The eukaryotic translation initiation factor 4E (eIF4E) protein is a vital component of the cap-dependent mechanism for mRNA translation. It binds the 7-methylguanosine (m7G) cap structure present at the 5′ end of mRNA molecules and recruits it as part of the eIF4F assembly which also includes two other partner proteins, eIF4A and eIF4G, to the translational machinery for protein synthesis. We have used a structure-guided approach to rationally develop a set of hydrocarbon stapled-peptides with high binding affinities and residence times against the oncogenic eukaryotic translation initiation factor 4E (eIF4E) protein. Crystal structures of these peptides in complex with eIF4E show that they form specific interactions with a region on the protein-binding interface of eIF4E which is distinct from the other well-established canonical interactions.

Two 15mer peptide derivatives of sTIP-05 (sTIP-09: 1KKRYSR*QLL*FRRR15 and sTIP-10: 1KKRYSREQLL*FQR*15) were synthesized, one with an “13RRR15” sequence extension and the other with an i, i + 4 hydrocarbon staple shifted to positions 11 and 15 of the peptide sequence which encapsulates the “12FQR14” sequence at the C-terminus. Significantly though, their rates of dissociation decreased relative to sTIP-05 and hence residence times were improved (68 seconds for sTIP-09 and 39 seconds for sTIP-10). The guanidinium group of R13 was involved in cation–pi interactions with residues W73, Y76 and hydrogen-bond interaction with the side-chain of N77. For R14, only the backbone atoms were visible while no clear density was seen for R15. We computationally generated a complete model of the sTIP-09 peptide using the crystal structure as a template and subjected the complex to MD simulations (Movie S5†). The simulated trajectory showed that R13 was relatively stable, remained in contact with the protein residues (albeit via an unstable R13–N77 hydrogen-bond, occupancy < 10%) and hence, contributed favorably (–2.2 kcal mol–1) to binding along with the other core residues (Y4, R6, L9, L10 and F12; –1.7 to –7.3 kcal mol–1) in the peptide. R14 and R15 did not interact stably with the protein and this was also reflected in the absence of any significant energetic contributions from these residues. They were highly dynamic, corroborating the lack of density in the crystal structure, similar to that seen for the “ButPhI” functional group in &13.

> EVANPEHYIKHPLQNRWALWFFKNDKSKTWQANLRLISKFDTVEDFWALYNHIQLSSNLMPGCDYSLFKDGIEPMWEDEKNKRGGRWLITLNKQQRRSDLDRFWLETLLCLIGESFDDYSDDVCGAVVNVRAKGDKIAIWTTECENREAVTHIGRVYKERLGLPPKIVIGYQSHADTATKSGSTTKNRFVV;> XKKRYSRLQLLLFRRR> GSGAMQNSQEMAITTLSLPKGGGAINGMGESVGQAGPDGMVTFSIPLPFSAGRGVAPALSLSYSSGAGNGPFGMGWQCSAMSISRRTQKGVPQYNEDDEFLSPSGEVMAIALNDSGFEDVRTANRLQGIPLPFSYKVTRYQPRLIQDFIKIEYWQPVKQTDGTPFWIIYSPDGQTHILGKNSHSRVANAENPSQIASWLLEETVTPTGEHIYYQYSGENQVNCTDAEIALHPQDSAQRYLARIDYGNISPQASLFVLDEELPNLTQWLFHLVFDYGERDISI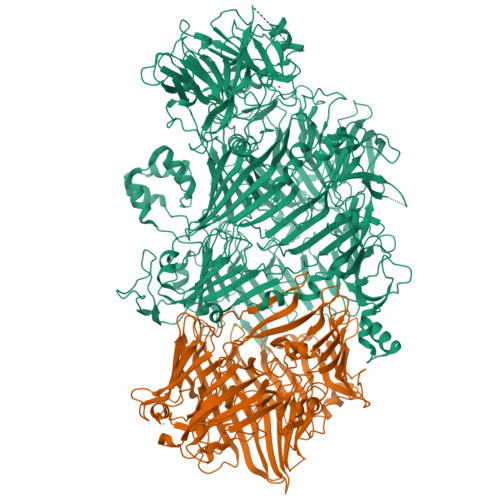NKIPTFEGGTTGWLARPDMFSRYDFGIEIRNRRLCHQVLGFHRLEALNDRDVTDEIPVLVNRLTLDYDLNNSVSTLVAVRQVAYETDGSPITQPPLEFDYQRFDTGSIPGWQEMPQLEAFNGYQPYQMIDLYGEGTPGILYQETPGAWWYKSPQRQIGGDSNAVTYGAMKALPKIPRLQEGATLMDINGDGRLDWVITSAGVRGFHSIHSTGEWTHFTPLNTLPTEYFHPKAQLADLVGAGLSDLVLIGPKSVRLYANQQGNWAPAQDVTQAENVSLPVIGIDSRQLVAFADMLGSGQQHLVEITADSVKCWPNMGHGRFGQPLTLEGFSQPQTSFNPDRVFLADIDGSGTNDIIYAHSECLEIYLNESGNRFSKPISLLLPDGVNFDNTCQLQAADIQGLGIASLVMTVPHMSPTHWRCDLALNKPWLLNVMNNNRGAETCLFYRSSAQFWLDEKQLVEAAGQQPECHLPFPMHLHWRSEIFDEITGNRLTQEQEYAHGSWDGQEREFRGFGRLIQRDTDGFAQGTVDIPTHPSRTVSWFATGIPEIDTTLSAEFWRGDDQAFSPFSPRFTRWENDSEAGSDVAFIPSEHDAFWLNRAMKGQLLRSELYGDDGTPEAEIPYSVTEMRHQVRALPTTDATVPSAWCSTIETRSYQYQRVAADPQCSQQVVIKADRYGSPLLSVAINYPRRKKPEKSPYPDDLPETLFDSSYDTQQQQLHLTKQQQNYFHLTNDDNWLLGLPKEQRNDGYQYDQERAPANGFTLETLIASNSLIGSNQPFTYLGQSRVAYQGGVDEQPSLQALVAYGETAILDEKTLQAFVGVLDSKTRDELLFSAGYQLAPRLFRVESEPDVWVARQGYSEFGDYSQFWRPLSQRSTLLTGKTTLKWDKHYCVVIETQDAAQLVTQARYDYRFLTPYSLTDANDNQHYVVLNPFGEVIASRFWGTEAGKDAGYSTPQAKPFVVPATIEAALALSPGIPVAHCAIFEPESWMQKLTQHDVSERMADNGTLWNALLQARFVTEDGYVCALGRRRWMARHGLSVLMLTLLAEIPRTPPHSLTITTDRYDSDDQQQLRQRILFSDGFGRLLQSAQRVEAGESWQRSEDSSLVVNVSGTPALVVTDNRWAVSGRTEYDGKGQGIRVYQPYFLDDWRYLSDDSARTDLFADTHIYDPLGREYQVITAKGYRRERQYTPWFVVNQDENDTAANLAI;> MSTSLFSRTPKVTVFDNRGLTARDIAYHRHPDAPEVTNERITPHQYDARGFLTQSADPRLHDAGRVNFSYLTDLAGGVLRTQGADNGTSVSLNDVAGRPFIVVSHISATDEGTEDRSLAVTRTWQYEDAALPGRPLNVTEQISTEVARITERFVYAGNTGAEKTLNLAGLCVRHYDTAGLVQTDSIALTGVSLSVTRRLLKDADNPDTVADWQGEGASAWNDLLSGEEYVTLTTADATGTVLTTTDAKGNIQRVRYDVAGLLSGSWLTVRDRTEQVIVKSLTYSAAGQKQREDHGNGVVITYTYEAETQRLTGIRTERPAGHASGAKVLQDLRYEYDPVGNVLKITNDAEATRFWSNQKVVPENTYTYDSLYQLVSATGREMANVGQQGSRLPSATVPFPTDSSAYTSYTRTYTYDEASNLTQIRHSPATRSGYTTNITVSNRSNRAVLSNLTENAADVDALFTAGGQQTQLQPGLGLVWTARNELLKVTPVMRDGSADDSENYRYDGGSQRILKVSVQKTGNSAQTQRALYLPGLELRSAKNGDTETESLQVITVGEASRAQVRMLHWESGRPDGITDDKVRYSYDNLTGSSVLELDSDGKLISMEEYYPYGGTAVWTVRSAVEANYKTVRYSGKERDATGLYYYGYRYYQPWAGRWLSADPAGSVDGLNLYRMVRNNPVAWKDNDGRIPINTMIPPPPPMMGGNPPPPPPMMGGNPPPPPPVAGGNPPPPPSMPGQQNGAKKNWVIKEDPALYKQQGGEYPYYSSFTIALQKLNISHYDSIIDMDNFISKWAEIGRNMKPAARDISHDKFIEVQKTLGKIDAEWSGYHSADVNETFRGDTPVISNSYSWLAEFINESEGKSDTVQKSMDLEIKSPLIMSTAKDPKMGYVSGKTIMWHFDLEPGHAGVSEGLYASEGEVTFPLYNRMKITSLQYLPEGRSYMDNPEQYGTSHRYIIKARMLPRS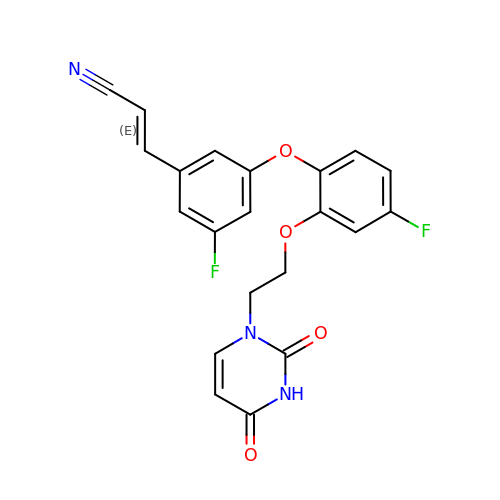(2E)-3-(3-{2-[2-(2,4-dioxo-3,4-dihydropyrimidin-1(2H)-yl)ethoxy]-4-fluorophenoxy}-5-fluorophenyl)prop-2-enenitrile | C21 H15 F2 N3 O4 | USRHSVZSPKDGMT-OWOJBTEDSA-N> GPGSMVTLQIDDDNRVRTLTLNRPEALNAFNEALYDATAQALLDAADDPQVAVVLLTGSGRGFSAGTDLAEMQARITDPNFSEGKFGFRGLIKALAGFP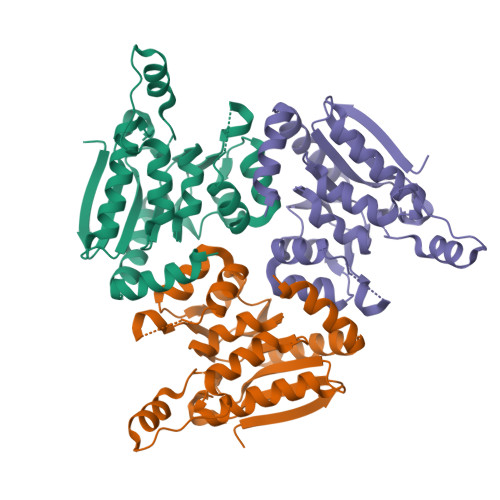KPLICAVNGLGVGIGATILGYADLAFMSSTARLKCPFTSLGVAPEAASSYLLPQLVGRQNAAWLLMSSEWIDAEEALRMGLVWRICSPEELLPEARRHAEILAAKPISSLMAVKHTMVEPNRAQIAAASARENAHFAELMGAQANAAALADFTDRRR2-(ACETYL-HYDROXY-AMINO)-4-METHYL-PENTANOIC ACID METHYL ESTER | C9 H17 N O4 | 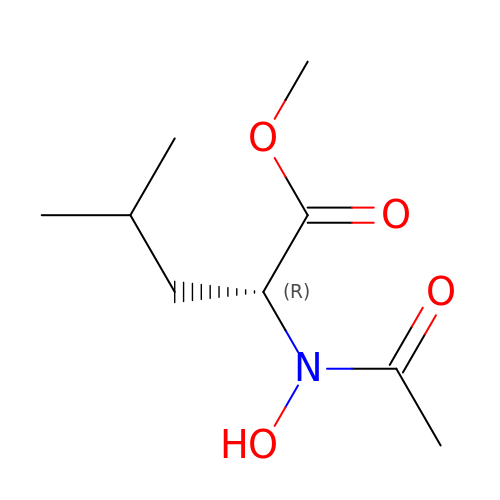OVUHENJPIUQHLJ-MRVPVSSYSA-N> SNAMSPATVLDSILEGVRADVAAREASVSLSEIKAAAAAAPPPLDVMAALR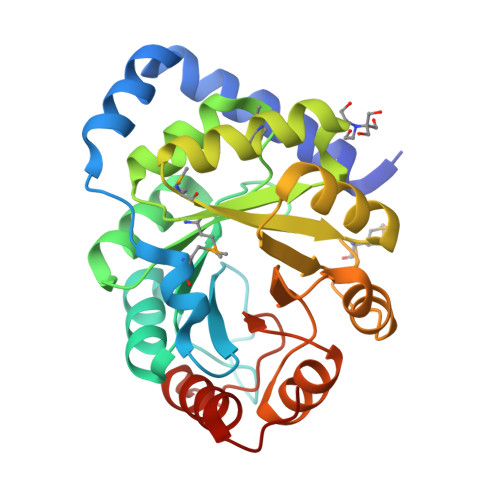EPGIGVIAEVKRASPSAGALATIADPAKLAQAYQDGGARIVSVVTEQRRFQGSLDDLDAVRASVSIPVLRKDFVVQPYQIHEARAHGADMLLLIVAALEQSVLVSMLDRTESLGMTALVEVHTEQEADRALKAGAKVIGVNARDLMTLDVDRDCFARIAPGLPSSVIRIAESGVRGTADLLAYAGAGADAVLVGEGLVTSGDPRAAVADLVTAGTHPSCPKPAR> MKQYLELMQKVLDEGTQKNDRTGTGTLSIFGHQMRFNLQDGFPLVTTKRCHLRSIIHELLWFLQGDTNIAYLHENNVTIWDEWADENGDLGPVYGKQWRAWPTPDGRHIDQITTVLNQLKNDPDSRRIIVSAWNVGELDKMALAPCHAFFQFYVADGKLSCQLYQRSCDVFLGLPFNIASYALLVHMMAQQC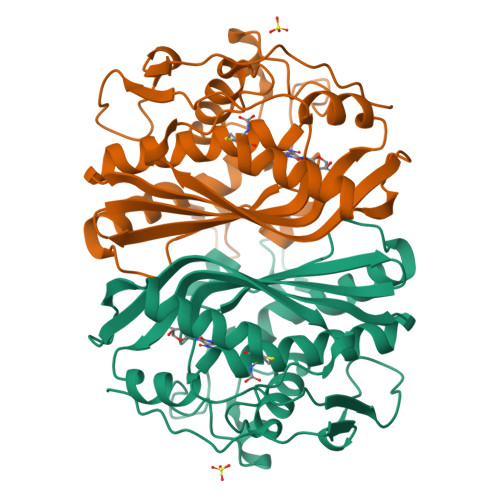DLEVGDFVWTGGDTHLMSNHMDQTHLQLSREPRPLPKLIIKRKPESIFDYRFEDFEIEGYDPHPGIKAPVAI> GSMSPVLTTPKRHAPPPEQLQNVTDFNYTPSHQKPFLQPQAGTTVTTHQDIKQIVEMTLGSEGVLNQAVKLPRGEDENEWLAVHCVDFYNQINMLYGSITEFCSPQTCPRMIATNEYEYLWAFQKGQPPVSVSAPKYVECLMRWCQDQFDDESLFPSKVTGTFPEGFIQRVIQPILRRLFRVYAH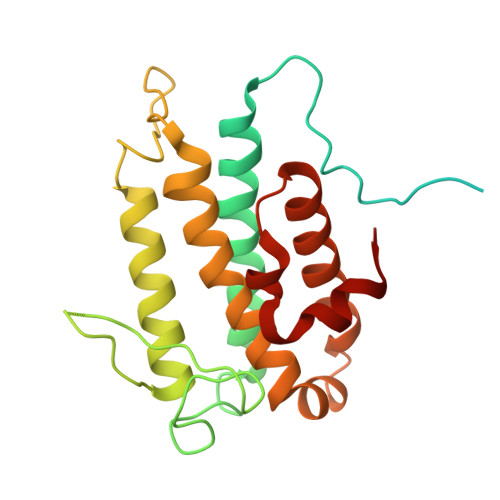IYCHHFNEILELNLQTVLNTSFRHFCLFAQEFELLRPADFGPLLELVMELRDR>[4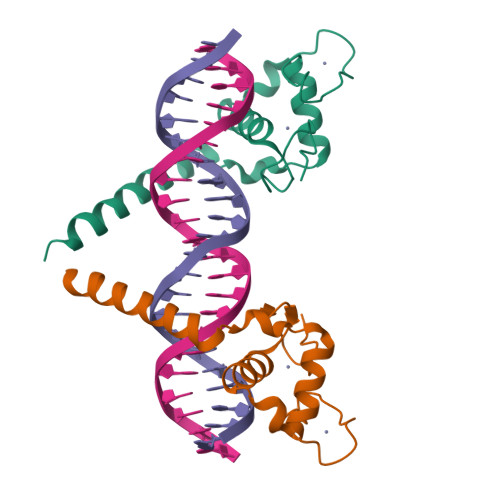x]GSDELCVVCGDKATGYHYRCITCEGCKGFFRRTIQKSLHPSYSCKYEGKCIIDKVTRNQCQECRFKKCIYVGMATDLVLDDSKRLAKRKLIEENREKRRREELQK>SNMDGRIVIVDDEPITRLDIRDIVIEAGYEVVGEAADGFEAIEVCKKTQPDLVLMDIQMPILDGLKAGKKIVQDQLASSIVFLSAYSDVQNTDKAKKLGALGYLVKPLDEKSLIPTIEMSIERGKQTQLLLSQIDKLSLKLEERKIIEKAKGILVKENHISEEEAYQMLRTLSMNKRARMSEIAELIVMDDE[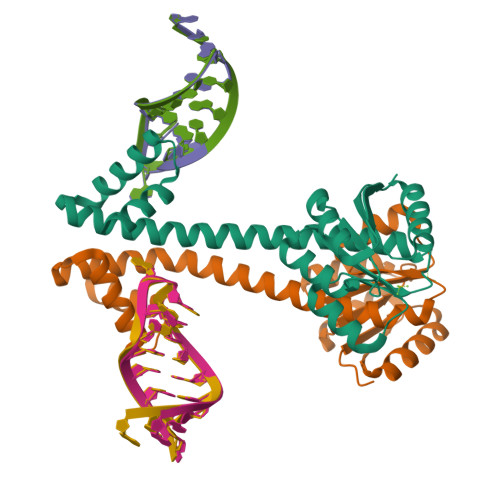2x]> ANIVGGIEYSINNASLCSVGFSVTRGATKGFVTAGHCGTVNATARIGGAVVGTFAARVFPGNDAAWVSLTSAQTLLPRVANGSSFVTVRG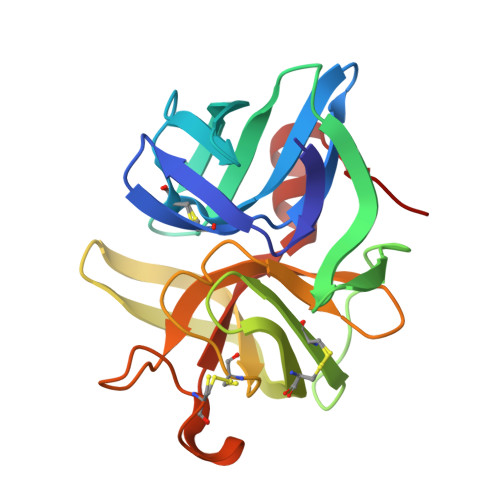STEAAVGAAVCRSGRTTGYQCGTITAKNVTANYAEGAVRGLTQGNACMGRGDSGGSWITSAGQAQGVMSGGNVQSNGNNCGIPASQRSSLFQRLQPILSQYGLSLVTG> MAFEFKLPDIGEGIHEGEIVKWFVKPGDEVNEDDVLCEVQNDKAVVEIPSPVKGKVLEILVPEGTVATVGQTLITLDAPGYENMTFKGQEQEEAKKEEKTETVSKEEKVDAVAPNAPAAEAEAGPNRRVIAMPSVRKYAREKGVDIRLVQGTGKNGRVLKEDIDAFLAGGAKPAPAAAEEKAAPAAAKPATTEGEFPETREKMSGIRRAIAKAMVHSKHTAPHVTLMDEADVTKLVAHRKKFKAIAAEKGIKLTFLPYVVKALVSALREYPVLNTSIDDETEEIIQKHYYNIGIAADTDRGLLVPVIKHADRKPIFALAQEINELAEKARDGKLTPGEMKGASCTITNIGSAGG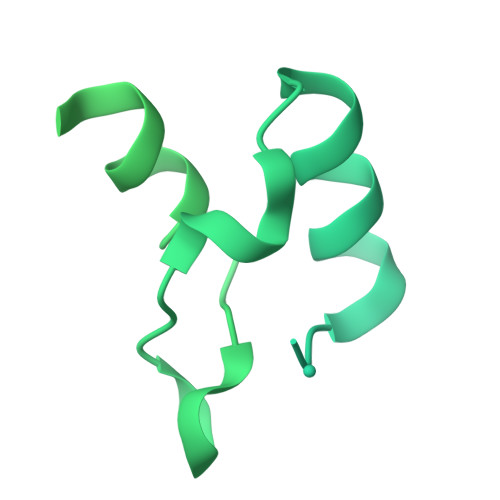QWFTPVINHPEVAILGIGRIAEKPIVRDGEIVAAPMLALSLSFDHRMIDGATAQKALNHIKRLLSDPELLLMEA>GYMLGSA[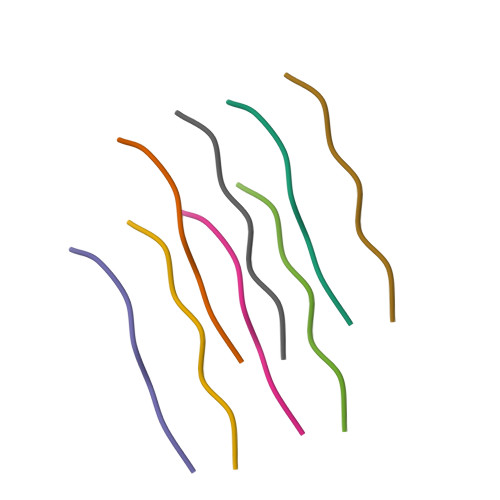2x]>[2x]MEKTREGKSSEAVSQWLTAFQLQLYAPNFISAGYDLPTISRMTPEDLTAIGVTKPGHRKKIAAEISGLSIPDWLPEHKPANLAVWLSMIGLAQYYKVLVDNGYENID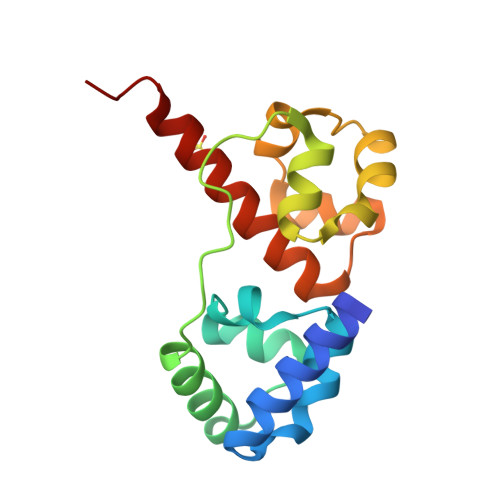FITDITWEDLQEIGITKLGHQKKLMLAVRKLAELRRHHHHHH In bacteria, uridine 1915 of the 23S rRNA undergoes two steps of post-transcriptional modification—pseudouridylation, followed by N3-methylation—that convert it to 3-methylpseudouridine (m3Ψ). RlmH acts on the assembled 70S ribosome. RlmH consists of five parallel β-strands (β2-β1-β4-β3-β5) sandwiched between two layers of α-helices: α2 and α4 on the solvent side, and α1, α5 and α3 on the dimerization interface. Our data suggest that E. coli RlmH functions as a dimer, with the SAM binding pocket of one monomer and the C-terminal residues of its counterpart forming a composite active site.

To gain insight into the mechanism of RlmH, we determined 2.3 and 2.1 Å X-ray structures of E. coli RlmH with the cofactor SAM and with the SAM-mimicking inhibitor sinefungin. The crystal structures of E. coli RlmH bound to the cofactor SAM or to the inhibitor sinefungin contain two dimers of RlmH in an asymmetric unit, with two cofactors bound to each RlmH dimer. Each of the two cofactors (SAM and sinefungin) binds to RlmH in a bent conformation in which the amino-acid moiety of the cofactor folds toward the adenine base. This conformation resembles that in other ligand-bound structures of SPOUT family members. Because the two cofactors adopt similar conformations, we focus our discussion on the structure bound to SAM.

>MHHHHHHVKLQLVAVGTKMPDWVQTGFTEYLRRFPKDMPFELIEIPAGKRGKNADIKRILDKEGEQMLAAAGKNRIVTLDIPGKPWDTPQLAAELERWKLDGRDVSLLIGGPEGLSPACKAAAEQSWSLSALTLPHPLVRVLVAESLYRAWSITTNHPYHRE[4x]> GAATGCGTAGCTGT;> CGGACAGCTACGCAT;> ACAC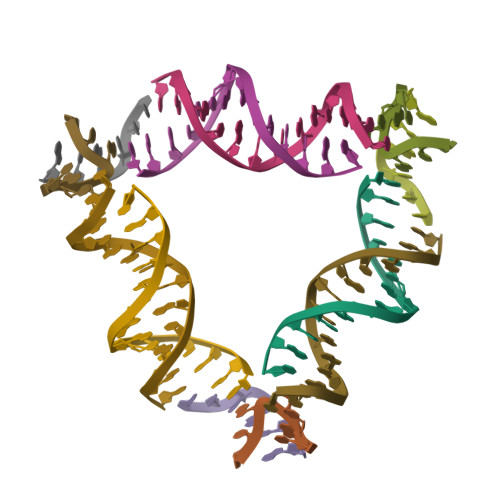CGT;> TCTGTA>[8x]MAVERTLIIVKPDAMEKGALGK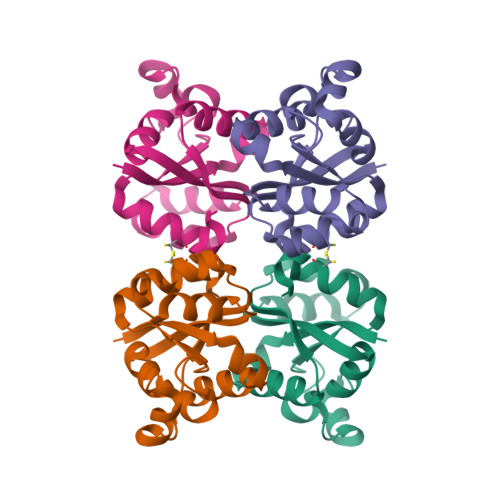ILDRFIQEGFQIKALKMFRFTPEKAGEFYYVHRERPFFQELVEFMSSGPVVAAVLEGEDAIKRVREIIGPTDSEEARKVAPNSIRAQFGTDKGKNAIHASDSPESAQYEICFIFSGLEIV> MDPFLVLLGSVSSSLSSSELTELKFLCLGRVGKRKLERVQSGLDLFSMLLEQNDLEPGHTELLRELLASLRRHDLLRRVDDFEAGAAAGAAPGEEDLCAAFNVICDNVGKDWRRLARQLKVSDTKIDS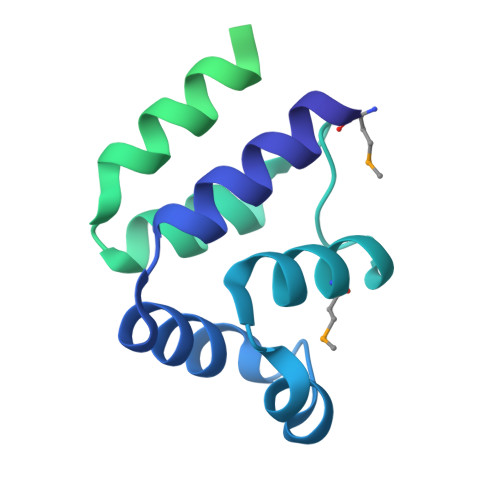IEDRYPRNLTERVRESLRIWKNTEKENATVAHLVGALRSCQMNLVADLVQEVQQARDLQNRSGAMSPMSWNSDASTSEASLEHHHHHH>GHMTTTPKPRTAPAVGSVFLGGPFRQLVDPRTGVMSSGDQNVFSRLIEHFESRGTTVYNAHRREAWGA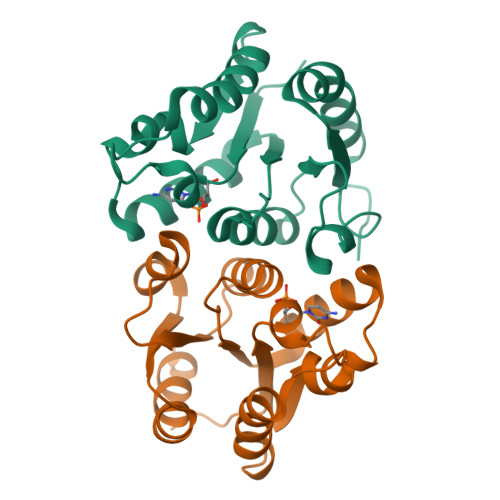EFLSPAEATRLDHDEIKAADVFVAFPGVPASPGTHVEIGWASGMGKPMVLLLERDEDYAFLVTGLESQANVEILRFSGTEEIVERLDGAVARVLGRAGEPTV[2x]>[2x]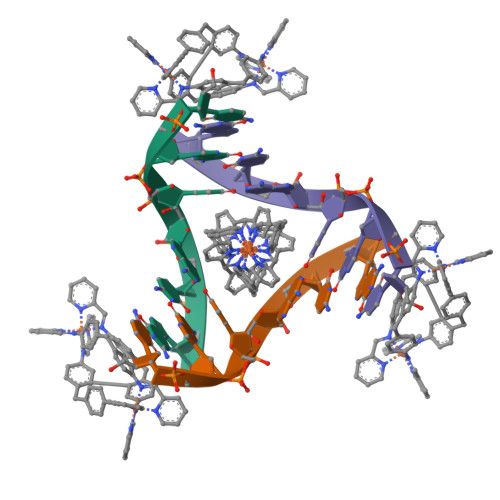CGTACG> MPSRTELLAEEYLRREGHDPQKFRYVHPDGTPYTDADGLARIARLAVPPAYQDVYVSPDAENELQA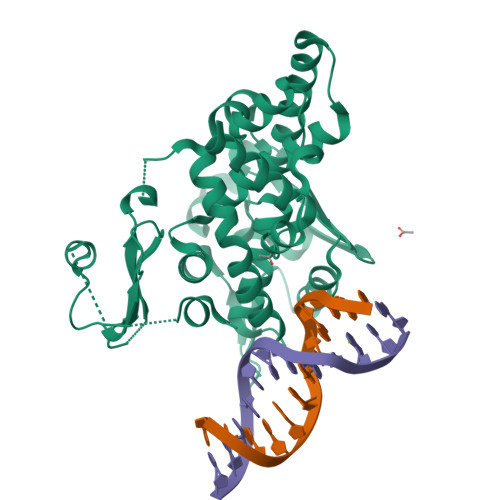FGRDAAGRLQYRYHPDFVQAGALKKWQRLTRFAGALPTLKVATTADLRASGLPPRKVMALMTRLLHVARFRVGSDIYARQHKTYGLSTLRQRHVVVDGNTVTFRFKGKHGVSQHKATSDRTLAANMQKLLDLPGPWLFQTVDAGGGERRRIHSTELNAYLREVIGPFTAKDFRTWGGTLLAAEYLAQQGTESSERQAKKVLVDCVKFVADDLGNTPAVTRGSYICPVIFDRYLDGKVLDDYEPRTERQEAELEGLTRSEGALKRMLESERTLRQRGRALK Acetyl Coenzyme A Carboxylase (ACC), an important enzyme that catalyzes the first reaction of fatty acid biosynthesis, is biotinylated by biotin acetyl-CoA carboxylase ligase (BirA). The Mtb-BirA molecule is composed of two domains; N-terminal domain 1 comprises of 7 β-strands (β1: 29–32, β2: 55–59, β3: 82–88, β4: 124–126, β5: 131–133, β6: 137–147 and β7: 150–158) and 6 α-helices (α1: 13–20, α2: 39–48, α3: 95–114, α4: 173–176, α5: 183–203, α6: 206–215), while C-terminal domain 2 is a SH3 domain with 5 strands forming an antiparallel β-sheet (β8: 220–227, β9: 231–240, β10: 246–250, β11: 253–257 and β12: 261–264). The two domains are linked together with loop L10 (216–219) that connects helix α6 of domain 1 and β8 strand of domain 2. All the apo BirA crystal structures have revealed the presence of disordered flexible loops, which undergo a conformational transition upon biotin and biotinyl-5′-AMP binding.

Hence, to eliminate the effects arising out of these differences, the Mtb-BirA structure (2.8 Å) was also determined with normal hydration for the purpose of comparison. Structures of dehydrated (dhMtb-BirA) and hydrated (hMtb-BirA) Mtb-BirA, were determined at 2.69 Å and 2.8 Å, respectively, using crystals grown under similar conditions. A noncrystallographic dyad exists between the two subunits in both hMtb-BirA and dhMtb-BirA structures. The pseudo-2-fold symmetric interface shared by two monomers of the asymmetric unit in both hMtb-BirA and dhMtb-BirA is ascribed to the C-terminal domain involving β11 strands and loops L11 (between β8–β9) and L13 (between β10–β11) of two monomers. The rmsds between the two subunits of dhMtb-BirA are 0.887 Å for 198 Cα equivalent atoms as opposed to the rmsds of 0.578 Å for 208 Cα pairs of the hMtb-BirA subunits. Two water molecules can be seen associated with residues P121 and D111 at the distance of 3.4 Å and 3.1 Å, respectively, in loop L6 of hMtb-BirA, whereas, these residues are no longer hydrated in dhMtb-BirA. The presence of water molecules in the hydrated structure keeps this loop in a closed-compact conformation.

>[2x]MTDRDRLRPPLDERSLRDQLIGAGSGWRQLDVVAQTGSTNADLLARAASGADIDGVVLIAEHQTAGRGRHGRGWAATARAQIILSVGVRVVDVPVQAWGWLSLAAGLAVLDSVAPLIAVPPAETGLKWPNDVLARGGKLAGILAEVAQPFVVLGVGLNVTQAPEEVDPDATSLLDLGVAAPDRNRIASRLLRELEARIIQWRNANPQLAADYRARSLTIGSRVRVELPGGQDVVGIARDIDDQGRLCLDVGGRTVVVSAGDVVHLR> MEVKYRGPSDDKLECEFLENNLLSCLREKSVQDNVAK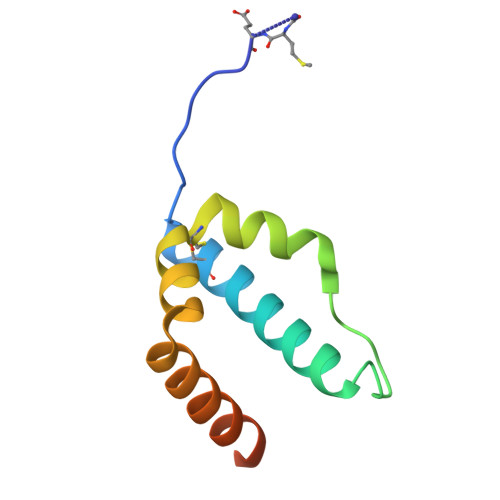MTCRPEFLVWFFLECPTKAAVYHDPKGLRNIFIQDKIKQKGSDDGVLSKDD> TGRPEWIWLALGTALMGLGTLYFLVKGM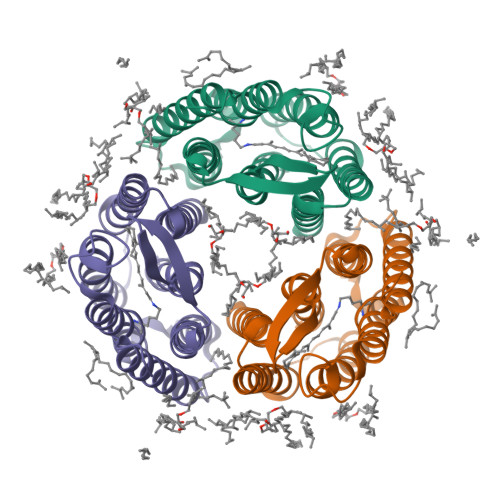GVSDPDAKKFYAITTLVPAIAFTMYLSMLLGYGLTMVPFGGEQNPIYWARYADWLFTTPLLLLDLALLVDADQGTILALVGADGIMIGTGLVGALTKVYSYRFVWWAISTAAMLYILYVLFFGFSMRPEVASTFKVLRNVTVVLWSAYPVVWLIGSEGAGIVPLNIETLLFMVLDVSAKVGFGLILLRSRAIFG> MPVKEGQAKLWFSTKEEADAYDDKMISNIELKSQDYEDENFSPVFNRKTQEYFLEPSEKFKSDFAELLRPLRSLSFNQVVDRYVLIPPNHTFYRNWTYEKFLGGFGLSYLILRELPLRNFYARVFVMYAF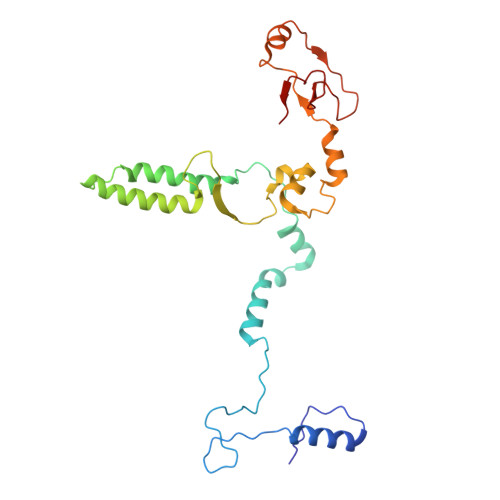AAKVLDHLGNPFPFSGHGQIVAAADRWNHWDVRCYDNVMKALKYIRIPTVQNNIPEATRWYGRQPGHLLRADTYWIPNLVSQRFAKHQPAHWDGTQNMPIFRLADPKHKDSYMVQFR>[2x]SNAMVMAPLPPVESLSLRQAIAQMIVVRGAGYLFDYERPYPQWEADQTTLQRWIEAGIGGVILLGGSAAEVAQKTKQLQSWAEIPLLIAADIEEGVGQRFRGATEFPPPMAFGEIWRTDPHQAIALAETMGATTAQEA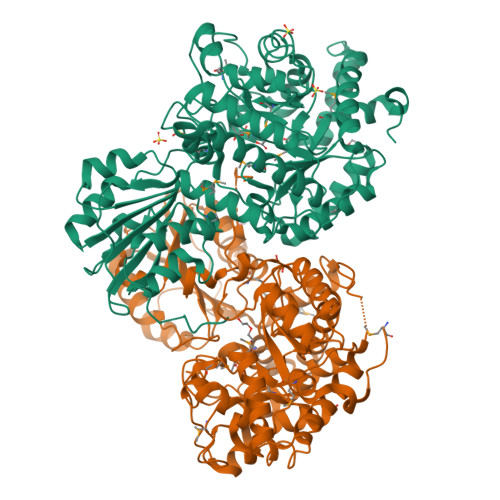LSLGINWVLAPVLDVNNNPHNPVINIRAFGETPDQVSALGTAFIRGAQQYAVLTTAKHFPGHGDTATDSHLALPTISHDDTRLNTVELPPFKAAIQGGVDAVMNAHLMIPAWDQQYPATLSPAILTGQLRHKLGFKGLIVTDALVMGGITQFAAPDTVVVQAIAAGADILLMPPDVDGAIIAIETAIKTGQLSESRIYESVERIWQAKQKILTATPSTFPQGISGDRPETRKTVAMVLERATKHQKSLVKISSFPDNFARNLIVVDSVLKSPFLRPNCPAIAIPQRHGYAAEIVELKTLPRLQLEAIPTLIQCFLRGNPFTEKLADPIDVLQKIAAQIPLQGVIFYGSPYFLEALQTTLPEIPWWFSYGQMAIAQAEICTSLWEEAPQAAPSAAEFI> MENMENDENIVVGPKPFYPIEEGSAGTQLRKYMERYAKLGAIAFTNAVTGVDYSYAEYLEKSCCLGKALQNYGLVVDGRIALCSENCEEFFIPVIAGLFIGVGVAPTNEIYTLRELVHSLGISKPTIVFSSKKGLDKVITVQKTVTTIKTIVILDSKVDYRGYQCLDTFIKRNTPPGYQASSFKTVEVDRKEQVALIMNSSGSTGLPKGVQLTHENIVTRFSHARDPIYGNQVSPGTAVLTVVPFHHGFGMFTTLGYLICGFRVVMLTKFDEETFLKTLQDYKCTNVILVPTLFAILNKSELLNKYDLSNLVEIASGGAPLSKEVGEAVARRFNLPGVRQGYGLTETTSAIIITPEGDDKPGASGKVVPLFKAKVIDLDTKKSLGPNRRGEVCVKGPMLMKGYVNNPEATKELIDEEGWLHTGDIGYYDEEKHFFIVDRLKSLIKYKGYQVPPAELESVLLQHPSIFDAGVAGVPDPVAGELPGAVVVLESGKNMTEKEVMDYVASQVSNAKRLRGGVRFVDEVPKGLTGKIDGRAIREILK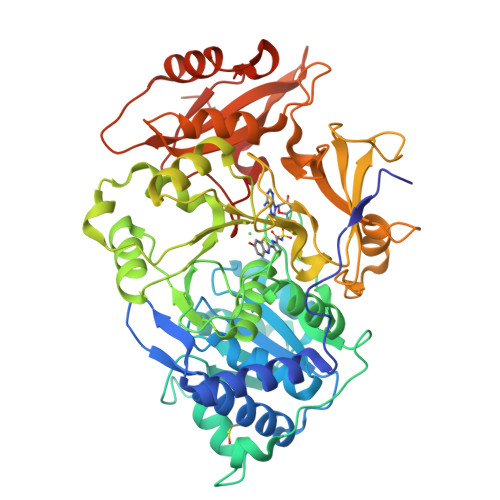KPVAKM> SLMERLGGGGFSARIFVGLN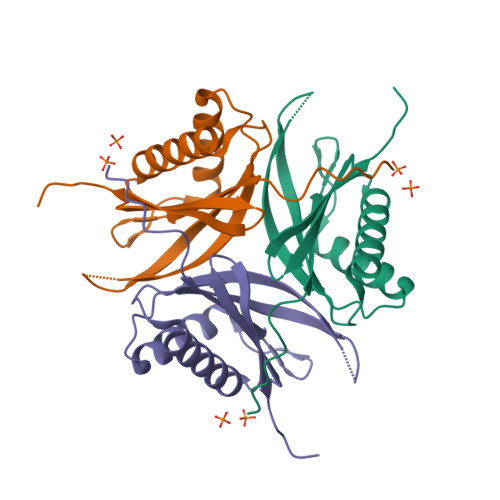VGDKPTYTIEDVVKDTIAIRKRQGILPDASFVAQRGVYTEQRSGQLVTENSVQIIIIDLEGLSKEDFTGKVQALGKELREDFKQESVIVEIQERGIVQDVYSITAEWYEEGPMRPLRVDLQPSLIS4-methylpyridazine | C5 H6 N2 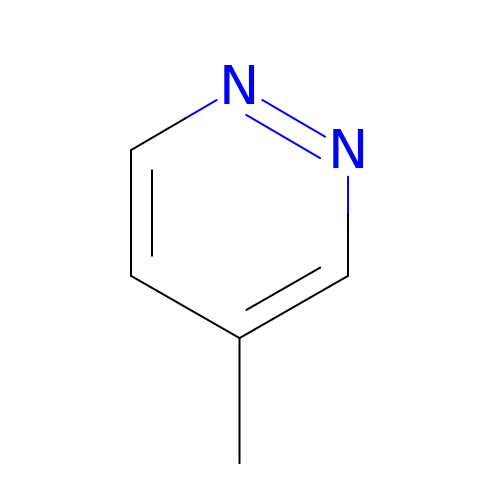| AIKUBOPKWKZULG-UHFFFAOYSA-N>GYVLGSA[2x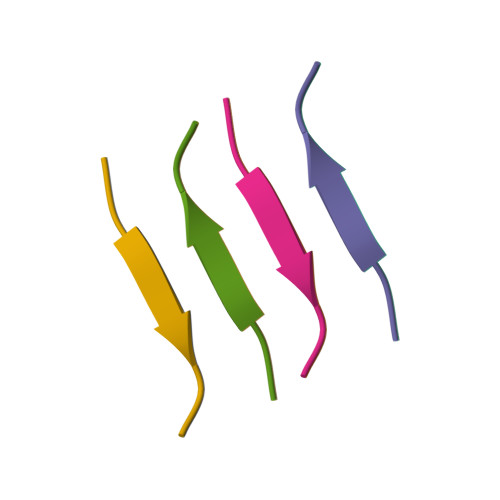]>MAFAKELFLGKIKKKEVFPFPEVSQDELNEINQFLGPVEKFFTEEVDSRKIDQEGKIPDETLEKLKSLGLFGLQVPEEYGGLGFSNTMYSRLGEIISMDGSITVTLAAHQAIGLKGIILAGTEEQKAKYLPKLASGEHIAAFCLTEPASGSDAAAIRSRATLSEDKKHYILNGSKVWITNGGLANIFTVFAKTEVVDSDGSVKDKITAFIVERDFGGVTNGKPEDKLGIRGSNTCEVHFENTKIPVENILGEVGDGFKVAMNILNSGRFSMGSVVAGLLKRLIEMTAEYACTRKQFNKRLSEFGLIQEKFALMAQKAYVMESMTYLTAGMLDQPGFPDCSIEAAMVKVFSSEAAWQCVSEALQILGGLGYTRDYPYERILRDTRILLIFEGTNEILRMYIALTGLQHAGRILTTRIHELKQAKVSTVMDTVGRRLRDSLGRTVDLGLTGNHGVVHPSLADSANKFEENTYCFGRTVETLLLRFGKTIMEEQLVLKRVANILINLYGMTAVLSRASRSIRIGLRNHDHEVLLANTFCVEAYLQNLFSLSQLDKYAPENLDEQIKKVSQQILEKRAYICAHPLDRTCHHHHHH[2x]

The Mitochondrial Complex I Assembly (MCIA) complex is essential for the biogenesis of respiratory Complex I (CI), the first enzyme in the respiratory chain, which has been linked to Alzheimer’s disease (AD) pathogenesis. Here we report the structural basis of the complex formation between the MCIA subunits ECSIT and ACAD9. ECSIT binding induces a major conformational change in the FAD-binding loop of ACAD9, releasing the FAD cofactor and converting ACAD9 from a fatty acid β-oxidation (FAO) enzyme to a CI assembly factor. The inclusion of an additional N-terminal 26 residues in the ECSIT construct (hereafter named ECSITCTER, residues 221–431), combined with optimisation of the purification and subcomplex reconstitution protocols led to a 3.0 Å resolution cryo-EM structure of the ACAD9WT-ECSITCTER complex, enabling us to build and refine an atomic model that includes nearly all ACAD9 residues as well as a 15-residue peptide spanning ECSIT residues 320–334. As previously described, ACAD9 is present as a dimer, where the C-terminal regions (residues 600–621) form helix loops that are positioned around the neighbouring protomer thereby stabilising the active dimer.

An ACAD9-S191A mutant further confirmed the lower affinity for ECSITCTER, though this mutant showed higher stability compared to ACAD9WT, with less dissociation into monomers. Considering the observed stability and compactness of the ACAD9S191A mutant, we chose it as a suitable candidate for further improving the ACAD9 structure. To increase the orientational diversity, we collected a 35° tilted cryo-EM data set and solved the structure of ACAD9S191A at 3.6 Å resolution. Consistent with FAO activity, the structure features one molecule of FAD in the cofactor binding site of each ACAD9 protomer. As expected, no significant density occupies the ECSIT binding site identified in the ACAD9WT-ECSITCTER structure. In particular, the structure of ACAD9S191A shows that this loop adopts a closed, downward facing position, forming hydrogen bonds with the α11-α12 loop of the neighbouring monomer and thereby acting as a barrier between the adenine nucleotide of the FAD molecule and the external solvent. Although it does not directly interact with the FAD molecule, we suggest that removal of this barrier destabilises the cofactor environment, leading to deflavination and the reassignment of ACAD9 from an FAO enzyme to a CI assembly factor. The downward facing loop position in ACAD9S191A clashes with the superposed ECSIT 310-helix indicating that the flipping mechanism is essential for ECSIT binding and MCIA formation. Similarly to the ACAD9WT-ECSITCTER dataset, residues 455-485 could not be built into the ACAD9S191A map.> MFQTFISRHNSNFFSDKLVLTSVTPASSAPVLQTPKATSSTLYFDSLTVNAGNGGFLHCIQMDTSVNAANQVVSVGADIAFDADPKFFACLVRFESSSVPTTLPTAYDVYPL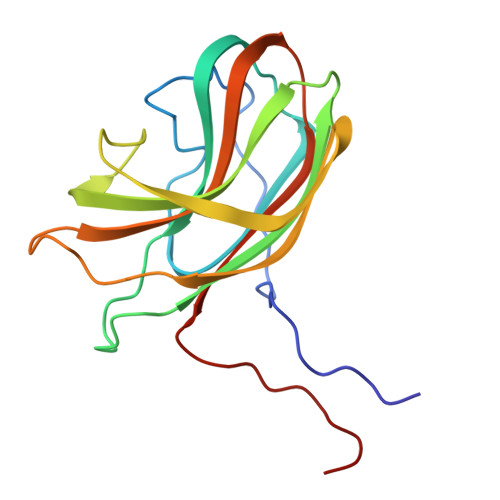NGRHDGGYYTVKDCVTIDVLPRTPGNNVYVGFMVWSNFTATKCRGLVSLNQVIKEIICLQPLK> SLFKDDIQLNEHQVAWYSKDWTAVQSAADSFKEKAENEFFEIIGAINNKTKCSIAQKDYSKFMVENALSQFPECMPAVYAMNLIGSGLSDEAHFNYLMAAVPRGKRYGKWAKLVEDSTEVLIIKLLAKRYQVNTNDAINYKSILTK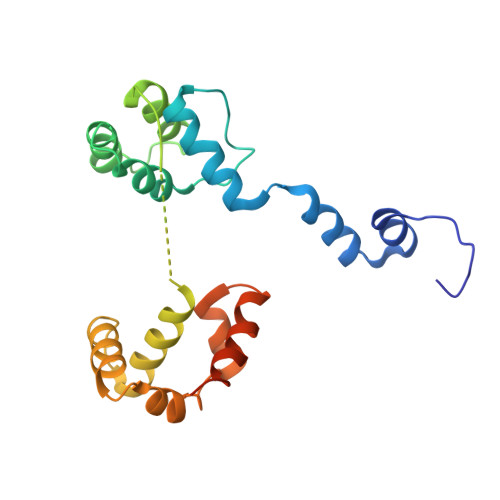NGKLPLVLKELKGLVTDDFLKEVTKNVKEQKQLKKLALEWGLEHHHHHHHHHH> MNKTKSEHIKQQALDLFTRLQFLLQKHDTIEPYQYVLDILETGISKTKHNQQTPERQARVVYNKIASQALVDKLHFTAEENKVLAAINELAHSQKGWGEFNMLDTTN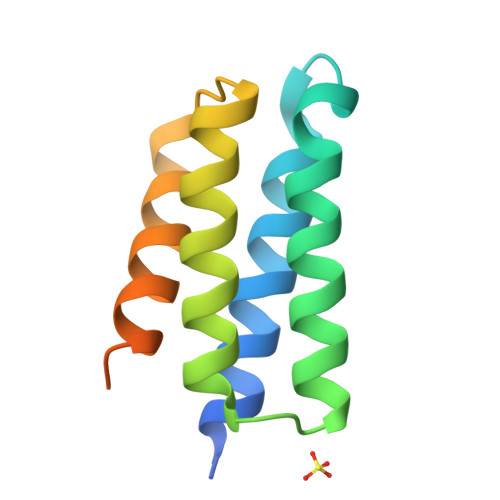TWPSQ>SMTDEYQLYEDIGKGAFSVVRRCVKLCTGHEYAAKIINTKKLSARDHQKLEREARICRLLKHSNIVRLHDSISEEGFHYLVFDLVTGGELFEDIVAREYYSEADASHCIQQILEAVLHCHQMGVVHRDLKPENLLLASKCKGAAVKLADFGLAIEVQGDQQAWFGFAGTPGYLSPEVLRKEAYGKPVDIWACGVILYILLVGYPPF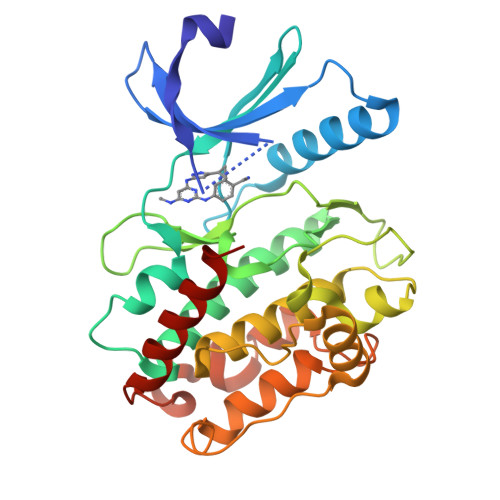WDEDQHKLYQQIKAGAYDFPSPEWDTVTPEAKNLINQMLTINPAKRITAHEALKHPWVCQRSTVASMMHRQETVECLKKFNARRKLKGA[4x]>KKRLTESQFQEAIQGLEVGQQTIEIARGVLVDGKPQATFATSLGLTRGAVSQAVHRVWAAFEDKNLPEGYARVTAVLPEHQAYIVRKWEADAKKKQ[2x];>[6x]KKRLTESQFQEAIQGLEVGQQTIEIARGVLVDGKPQATFATSLGLTRGAVSQAVHRVWAAFEDKN

Gene expression in the IncP-1 plasmids is stringently controlled by a network of four global repressors, KorA, KorB, TrbA and KorC interacting cooperatively. KorA is a 101-amino acid, homodimeric, protein with an N-terminal DNA-binding domain (DBD), containing a helix-turn-helix motif, and a C-terminal dimerization region, joined by a linker of four amino acids. In this study, we have determined the structures of the free KorA repressor and two complexes each bound to a 20-bp palindromic DNA duplex containing its consensus operator sequence. The structure of KorA consists of two domains, joined by a highly flexible, four amino acid linker, which retains its mobility even when bound to DNA.

KorA was crystallized in the presence of the operator OA. In contrast to the free protein, several crystal forms of the complex were obtained. Structures from two of these were determined. Both show the DBDs of the protein symmetrically placed about the DNA axis. In contrast, the orientation of the CTD differs in the two crystal structures. However, only one CTD could be modelled, although all eight DBDs are clearly visible. There is only weak, partial electron density for the other three CTDs, presumably as they are highly disordered. In contrast to most proteins containing a helix-turn-helix motif, that bind to one face of the DNA; the two DBDs of KorA straddle the DNA, with helix 4 of the two subunits binding to opposite faces of the major groove. In addition, the recognition helix of KorA, helix 4, is longer than in classical helix-turn-helix proteins and so the CTD is held away from the operator DNA and it has no interactions with the DBDs, making it flexible even in the presence of DNA. Given the highly flexible structure of the protein, MD simulations were used to explore the conformations of the free and bound protein in solution. Figure 5 shows an overlay of the conformers sampled for the KorA–DNA complex, over 100 ns of simulation; the complex remains very flexible with the CTD exploring a wider range of orientations than the two observed in the crystal structures.> ARVTVQDAVEKIGNRFDLVLVAARRARQMQVGGKDPLVPEENDKTTVIALREIEEGLINN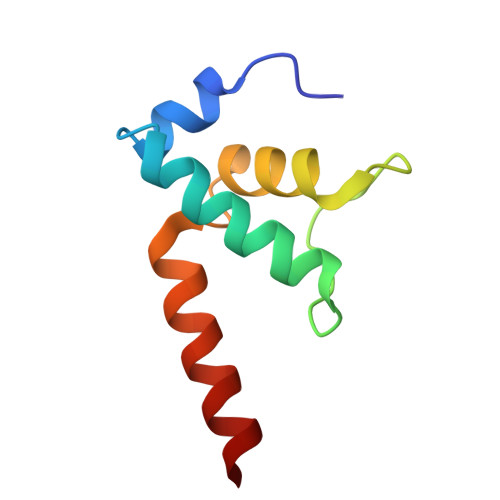QILDVRERQEQQEQEA> GSKEGEYIKLKVIGQDSSEIHFKVKMTT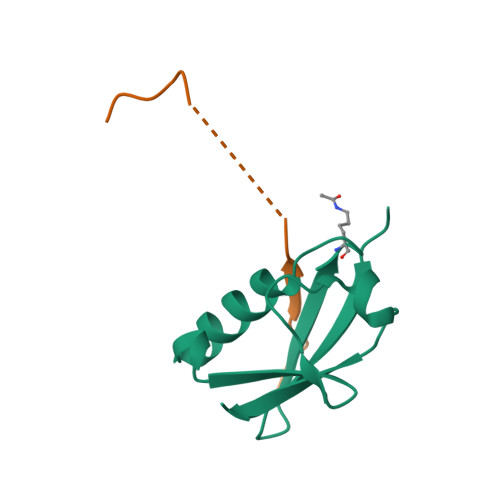HLKKLKESYAQRQGVPMNSLRFLFEGQRIADNHTPKELGMEEEDVIEVYQEQTGG;> GSGAGEAEERVVVISSSEDSDAENSSSRY CYMAL-4 | C22 H40 O11 | 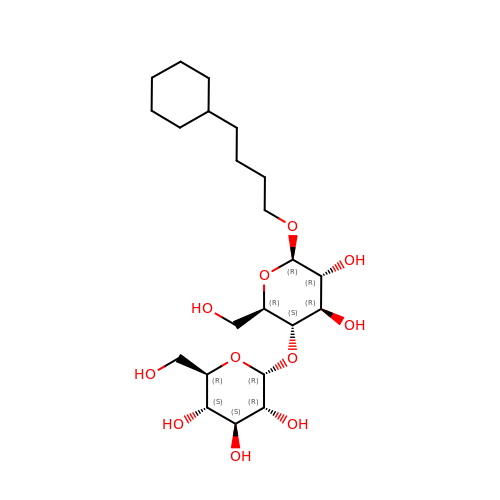JRNQXDHDSXBSFV-WXFJLFHKSA-N>MQVNRLPFFTNHFFDTYLLISEDTPVGSSVTQLLARDMDNDPLVFGVSGEEAS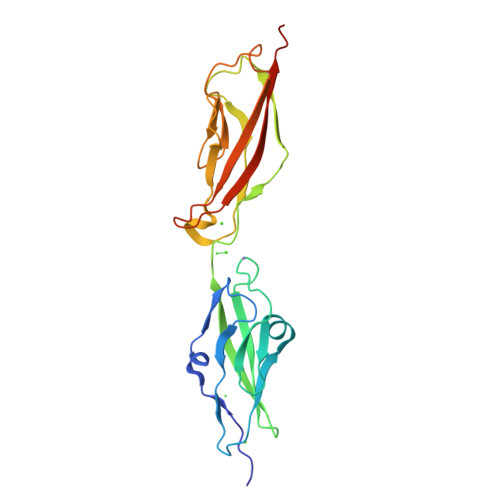RFFAVEPDTGVVWLRQPLDRETKSEFTVEFSVSDHQGVITRKVNIQVGGVNDNAPTFHNQPYSVRIPENTPVGTPIFIVNATDPDLGAGGSVLYSFQPPSPFFAIDSARGIVTVIQELDYEVTQAYQLTVNATDQDKTRPLSTLANLAIIITDLEHHHHHH[2x]> SNAADSVVPAGETVNGGTLINHDRQFVSGTADGMTVSTGLELGADSDNNTGGQQIARGGTARNTRVTA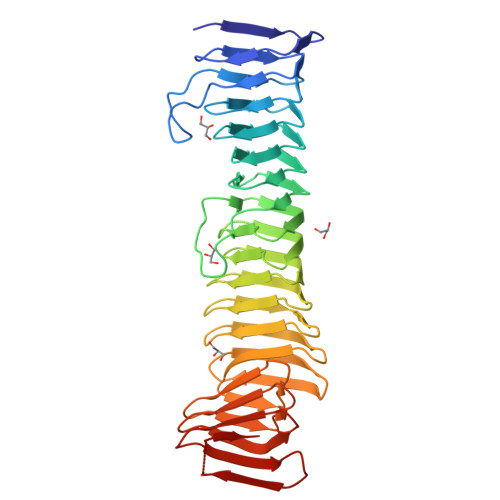NGLQDVMAGGSTSDTVISTGGGQNLRGKASGTVLNDGDQWIHAGGRASGTVINQDGYQTIKHGGLVTGTIVNTGAEGGPDSENVSTGQMVGGIAESTTINKNGRQVIWSSGIARDTLIYTGGDQTVHGEAHNTRLEGGNQYVHKYGLALNTVINEGGWQVVKAGGTAGNTTINQNGELRVHAGGEASDVTQNTGGALVTSTAATVTGTNRLGAFSVVEGKADNVVLENGGRLDVLSGHTATRTLVDDGGTLDVRNGGTATAVSMGNGGVLLADSGAAVSGTRSDGTAFRIGGGQADALM>FLKSXALL[2x]

Novo29 is an eight-residue depsipeptide comprising a macrolactone ring and a linear tail. Novo29 kills bacteria by inhibiting bacterial cell-wall synthesis, with no detectable resistance occurring upon serial passaging. We also report the X-ray crystallographic structure of a hydroxyAsn epimer of Novo29 (epi-Novo29), which may provide insights into how Novo29 binds bacterial cell-wall precursors.

The crystallographic phases of the higher-resolution data were determined by molecular replacement using the KI-soaked structure as a search model. The asymmetric unit contains two molecules of epi-Novo29, which exhibit only minor differences in conformation. In the X-ray crystallographic structure, epi-Novo29 adopts an amphiphilic conformation, with the side chains of Phe1, d-Leu2, Leu7, and Leu8 creating a hydrophobic surface and the side chains of d-Lys3, Ser4, and (2R,3S)-hydroxyAsn5, as well as the N-terminal ammonium group, creating a hydrophilic surface. An intramolecular hydrogen bond between the main-chain NH group of Ala6 and the side chain OH group of Ser4 helps enforce this conformation. In the lattice, epi-Novo29 packs so that the hydrophobic surfaces come together, with four sets of epi-Novo29 molecules forming a hydrophobic core. The macrolactone ring of epi-Novo29 adopts a conformation in which the main-chain NH groups of (2R,3S)-hydroxyAsn5, Ala6, Leu7, and Leu8 converge to create a cavity, which binds ordered water and acetate anion. Although epi-Novo29 is much smaller than PSMα3 (8 residues instead of 22 residues) the epi-Novo29 molecules daisy-chain through intermolecular hydrogen bonding to form extended structures that resemble the larger α-helices of PSMα3. In contrast, epi-Novo29 exhibited no MIC activity (>32 μg/mL) against any of the bacteria, thus indicating that the 2R,3R stereochemistry of the hydroxyAsn residue is critical to the antibiotic activity of Novo29. Inversion of the 3S-stereocenter of the (2R,3S)-hydroxyAsn residue of the crystal structure, followed by geometry optimization of only the side chain of the resulting (2R,3R)-hydroxyAsn residue, afforded a crystallographically based molecular model of Novo29. The only difference in structure is that the side-chain amide NH group of the (2R,3R)-hydroxyAsn residue hydrogen bonds to the carbonyl group of Phe1.Each protein forms key interactions to promote cell infection, with the terminal domain of the fiber, the fiber knob protein, interacting with the viruses’ primary cell entry receptor. The adenovirus fiber knob protein is known to have a highly conserved trimeric structure. Sialic acid (SA) usage has been proposed as a cell infection mechanism for EKC causing HAdV-D. Here we highlight an important role for SA engagement by many HAdV-D. We provide apo state crystal structures of 7 previously undetermined HAdV-D fiber-knob proteins, and structures of HAdV-D25, D29, D30 and D53 fiber-knob proteins in complex with SA. Our findings demonstrate a conserved binding site for sialic acid, common across the species D adenoviruses, therefore suggesting that, along with CAR, the receptor can be used to initiate cell entry.

HAdV-D15, D24 and D32 were crystallised in only their apo states, whereas HAdV-D25, D29, D30 and D53 crystals were also soaked with sialic acid. To evaluate the potential for these recombinant fiber knob proteins to bind cellular sialic acid residues, crystals of the fiber-knob proteins were also soaked with sialic acid prior to data collection. This resulted in four structures of HAdV-D25, D29, D30 and D53 in complex with sialic acid also shown in Fig. 1. The conformation of the bound sialic acid was found to be a mixture of the α and β anomers, freely exchangeable in solution and minimal protein side chain adjustment was required to accommodate either conformation. Soaking in sialic acid containing solutions reduced resolution slightly. Whilst the threonine was not found to be universally conserved, the other species D adenoviruses had similar sized residues which generally made interactions with sialic acid in HAdV-D29, D30 and D53. However, the four sialic acid soaked novel crystal structures, provide a much more reliable view of the binding pocket and interactions with sialic acid.

>[3x]NDKLTLWTTPDPSPNCKVSEEKDSKLTLVLTKCGSQILASVSLLVVKGKFANINNETNPGEDYKKFSVKLLFDANGKLLTGSSLDGNYWNYKNKDSVIGSPYENAVPFMPNSTAYPKIINNGTANPEDKKSAAKKTIVTNVYLGGDAGQPVATTVSFNKETESNCVYSITFDFAWNKTYKNVPFDSSSLTFSYIAQDAEDKNE Cystatins are inhibitors specifically controlling the activity of cysteine proteases. The cystatin superfamily shares a common fold that is characterized by a 5-stranded antiparallel β-sheet that is enwrapping a central α-helix. Because of its strict specificity for cleaving after asparagine residues, it is synonymously referred to as the asparaginyl-endopeptidase (AEP)2 (15, 16). This strict preference is exploited by the legumain-inhibitory cystatins C, E, and F, which use a conserved Asn39 residue, localized on a reactive center loop different from the papain-inhibitory site to specifically bind to the legumain active site. Cystatin E is the most potent physiologic legumain inhibitor, binding 100-fold more tightly as compared with cystatin C. Thereby, it is associated with a tumor suppressor function in prostate cancer, melanoma, and oral carcinoma cells.

From a structural perspective, the hCE dimer was assembled from two hCE monomer conformers that are connected via their L1 loops. Analysis with PDBePISA and PDBsum revealed that the hCE dimer interface is built up by 45 hydrogen bonds, 361 nonbonded contacts, and two charge-driven interactions. This results in a buried surface area of the dimer interface of 6710 Å2 and an interface area of ∼3354 Å2. Furthermore, the free energy of complex dissociation, ΔGdiss, of 55.4 kcal/m indicates that the dimer is thermodynamically stable. Remarkably, we discovered the assembly of two hCE dimers to a tetramer. Nevertheless, the overall assembly (nearly parallel β2-β3 strands) is similar between stefin B, cystatin C, and cystatin E and therefore suggests a conserved mechanism of oligomerization. The dimers interact via hydrophobic contacts involving residues of the former L1 loops. Despite this large structural rearrangement, the local conformations of the legumain RCL and LEL were virtually identical in monomeric and dimeric hCE structures. The crystal structure of dimeric hCE uncovered two symmetric and functional legumain-binding sites, either of which is accessible for legumain binding. Upon dimerization, the L1 loop, which is essential for binding to the papain S1′ site, was incorporated into the newly formed βII-βIII sheet. Thus, loop L1 is not available for binding anymore, and the papain-inhibitory site is destroyed by the dimer interface.

>MDRPQERMVGELRDLSPDDPQVQKAAQAAVASYNMGSNSIYYFRDTHIIKAQSQLVAGIKYFLTMEMGSTDCRKTRVTGDHVDLTTCPLAAGAQQEKLRCDFEVLVVPWQNSSQLLKHNCVQMLEHHHHHH[2x]>MDVTCWKYAIPGEPGGELTAEEVFASKDTAFPEGFLWGAATAAYQIEGAAAEDGRGPSMWDTFSKIPGKIDNGDTGDVACDHYHRYKEDVKLMKGMGLKSYRFSVSWSRVLPEGTGAINPKGMEFYQNLTNELIANGIVPTVTLYHWDLPEALSKNGGWLNEDTAVAFGQYADVMFQALGDRVKLWFTLNEPWTTAIAGYGQGGHAPGLKNMAENPYMAGHNQLLGHAAAVKVYREKYQEKQGGKIGAVLSTEWKEPLCHTQEDKDAAERSLIWYLAWFADPIYKGDYPEEMKERVGDRMPAFTEQQKQDLKGSADFFGINHYATNLLQGPTEKIGAENYFSDLNGWIMMDPRWAVGDASWLSVVPWGMRRLLRWIKHRYDDPVVYVTENGLSVPNESAMTPEAALNDKMRVDYLQGYVAEMWKAINYDKVKVAGYY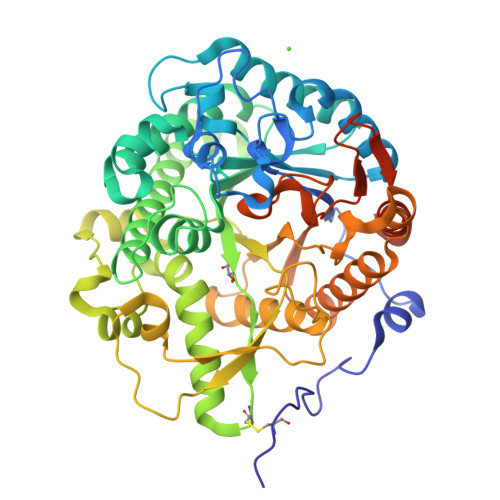HWSLLDNFEWSDGYKVRFGLVQVDYKTQKRTLKESAKVYKDMIAKYSGDTAPPDDAEAVARDAVKATPSAEAPLEHHHHHH[4x]> GSMSNINQMPREEGIDSTWRLMEEGYMYILNRRHSFNSDIFETRLLGKKAICMGGKEAAEIFYDTEKFKRKDAAPNRVVQTLFGKNGVQALDGQTHKHRKEMFMSIMSPDELEKLTDITKKQWEIAVDKWEQMDKVILYEEAKEIMCRTACQWAGVPVQENEVKRLTKNLGAMFESAAAVGLKHWLGRHARNYEEIWIEELIDRVRDGKVNPPENTTLHKFSWYRDLEGNLLDTETAAVEVINILRPIVAI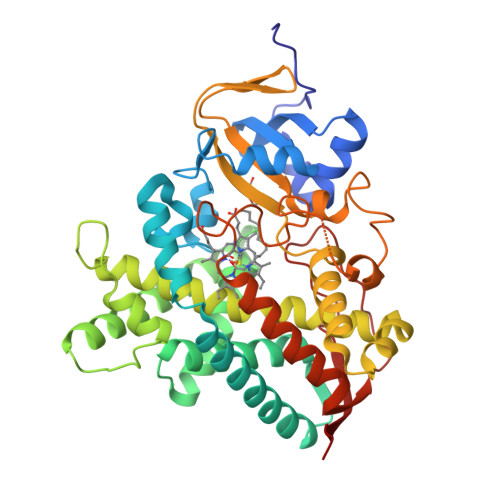AIFINFIALALHHYPEEKEKLKSGDKKYSQMFVQEVRRFYPFFPFVVALVKKDFTWKGYKFEEGTLTLLDLYGTNHDPEIWKNPDVFSPDRFAKWEGSPFSFIPQGGGDYFMGHRCAGEWVTIEVMKVSLDYLTNRMDYEVPDQDLSFSMASMPSIPHSKVVIKNVKKRI> MNIFRLTGDLSHLAAIIILLLKIWKSRSCAGISGKSQL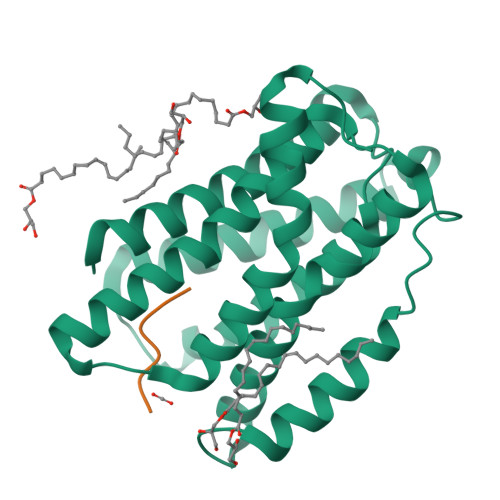LFALVFTTRYLDLFTSFISLYNTSMKLIYIACSYATVYLIYMKFKATYDGNHDTFRVEFLIVPVGGLSFLVNHDFSPLEILWTFSIYLESVAILPQLFMISKTGEAETITTHYLFFLGLYRALYLVNWIWRYYFEGFFDLIAVVAGVVQTVLYCDFFYLYVTKVLKGKKLSLPA;> TAEHDEL Curli, a prototypical functional amyloid formed by IDPs, serves a pivotal role in bacteria. Curli fibrils, widely expressed by Enteric bacteria like Escherichia coli and Salmonella spp., integrate into the extracellular matrix, promoting structural scaffolding, adhesion, and host colonization. The curli system consists of seven proteins encoded by two discrete operons (csgBAC and csgDEFG), which regulate the assembly of a major structural subunit, CsgA, and a minor subunit, CsgB, into curli fibrils. Using cryo-EM, we have shed the first light on the cryo-EM structure of E. coli CsgA fibrils, revealing that the amylogenic regions of CsgA adopt non-centrosymmetric beta-helical structures.

We chose an engineered CsgA with two designed cysteines (A63C and V140C), developed by Balistreri et al., as this selection offers several advantages for structural analysis. The final CsgA fibrils for cryo-EM imaging were formed in 10 mM CAPS buffer with 0.01% Tween 20, pH 10.4, without shaking, and heated at 70°C for 30 min. The chosen box size corresponds to the number of included CsgA monomers (the length of the fibril) for generating 3D models. Acceptable initial 3D models were generated by using box sizes of 218 and 260 pixels. The overall architecture of CsgA fibrils illustrated that seven and eight CsgA subunits could be assigned to the map of 218-pixel and 260-pixel box size, respectively. Fibrils comprising approximately 7–8 CsgA monomers appeared to exhibit high stability and uniformity, potentially indicating a characteristic of CsgA aggregation. The CsgA fibrils model indicated that the adjacent strand distance and helix height are approximately 4.8 Å and 19.1 Å, respectively, exhibiting the closest agreement with those (4.8 Å and 19 Å) shown in the predicted CsgA model. In addition, our E. coli CsgA models also confirmed the previous prediction that the core-facing residues between beta strands are imperfect repeats, leading to the formation of steric zippers that are non-centrosymmetric. Additionally, a central slice of the CsgA fibril map in three orthogonal projections revealed some additional density on both sides of the fibrils, likely attributed to the flexible N22 region. Due to the limit of map quality as a result of preferred orientation, the real resolutions (around 4–6 Å) are lower than the reported values (3.6–3.8 Å) by cryoSPARC, and therefore, the detailed interactions between these molecules within a fibril need to be revealed by further higher-resolution structures.

>MGVVPQYGGGGNHGGGGNNSGPNSELNIYQYGGGNSALALQTDCRNSDLTITQHGGGNGADVGQGSDDSSIDLTQRGFGNSATLDQWNGKNSEMTVKQFGGGNGAAVDQTASNSSVNVTQCGFGNNATAHQYHHHHHH[7x]> YAEHKSHRGEY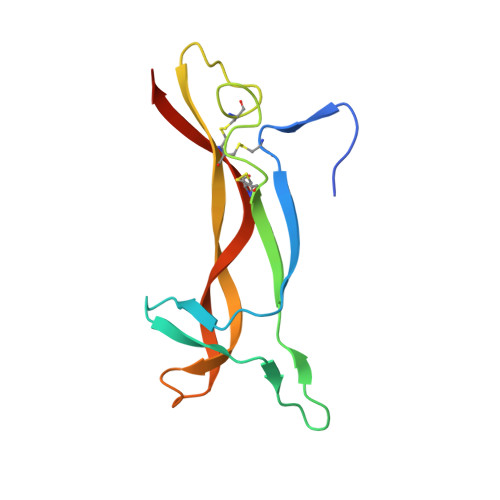SVCDSESLWVTDKSSAIDIRGHQVTVLGEIKTGNSPVKQYFYETRCKEARPVKNGCRGIDDKHWNSQCKTSQTYVRALTSENNKLVGWRWIRIDTSCVCALSRKIGRT> GHMERLLDELTLEGVARYMQSERCRRVICLVGAGISTSAGIPDFRSPSTGLYDNLEKYHLPYPEAIFEISYFKKHPEPFFALAKELYPGQFKPTICHYFMRLLKDKGLLLRCYTQNIDTLERIAGLEQEDLVEAHGTFYTSHCVSASCRHEYPLSWMKEKIFSEVTPKCEDCQSLVKPDIVFFGESLPARFFSCMQSDFLKVDLLLVMGTSLQVQPFASLISKAPLSTPRLLINKEKAGQSDPFLGMIMGLGGGMDFDSKKAYRDVAWLGECDQGCLALAELLGWKKELEDLVRREHASIDAQS

NAD+-dependent protein deacylases (sirtuins) constitute a unique class of enzymes that are conserved from bacteria to humans. The human isotype Sirtuin 2 (Sirt2) deacetylates both nuclear and cytoplasmatic proteins and thereby functions as a major cell cycle regulator, a determinant of myelination, a regulator of autophagy and a suppressor of brain inflammation. In this work, we present the first crystal structures of Sirt2 in complex with a potent and Sirt2-selective small-molecule inhibitor with drug-like properties.

We solved the structure of Sirt2 in complex with SirReal2 and the cosubstrate NAD+ (structure termed Sirt2–SirReal2–NAD+) as well as in complex with SirReal2 and an acetyl-lysine peptide derived from histone H3 (residues 11–17, structure termed Sirt2–SirReal2-H3). Both Sirt2–SirReal2 crystals belonged to different monoclinic space groups and contained one monomer per asymmetric unit. The position of SirReal2 in the EC-site of Sirt2 is very similar in both structures with either NAD+ or the acetyl-lysine peptide substrate (r.m.s.d. of 0.47 Å), and we will primarily describe the binding of SirReal2 in the presence of NAD+, as this structure likely represents the SirReal2-inhibited form of the enzyme. The aminothiazole SirReal2 occupies this EC-site adjacent to the C-pocket, which is the physiological site for product inhibition by the feedback inhibitor NCA30. The naphthyl moiety of SirReal2 protrudes into the substrate channel and the dimethylmercaptopyrimidine substituent (DMP) induces the formation of a binding pocket beyond the EC-site. The naphthyl moiety of SirReal2 that protrudes into the acetyl-lysine-binding site is in van-der-Waals contacts with the NCA moiety of NAD+, Phe131, Leu134, Ile169, Ile232, Val233 and Phe234. In the selectivity pocket, the DMP moiety forms π–π-stacking interactions with Tyr139 and Phe190 in the selectivity pocket that is shaped by Ile93, Ala135, Leu138, Pro140, Phe143, Leu206 and Ile213. In addition, Pro94 hydrogen bonds via a structural water molecule (W40) to the carbonyl-O of SirReal2. NAD+ of Sirt2–SirReal2–NAD+ also adopts a kinked conformation with a similar network of hydrophilic and hydrophobic interactions as observed for NAD+ or Carba-NAD+ in ternary sirtuin complexes (PDB-ID 2H4F34, Sir2Tm-Ac-Lys-p53-peptide-NAD+, PDB-ID 4FVT23, Sirt3-Carba-NAD+-Ac-Lys-ACS-peptide). The binding mode of NAD+ in Sirt2–SirReal2–NAD+ therefore shares a higher resemblance to the conformation of NAD+ in the ternary complex with Sir2Tm.> MHHHHHHPEIVDTCSLASPASVCRTKHLHLRCSVDFTRRTLTGTAALTVQSQEDNLRSLVLDTKDLTIEKVVINGQEVKYALGE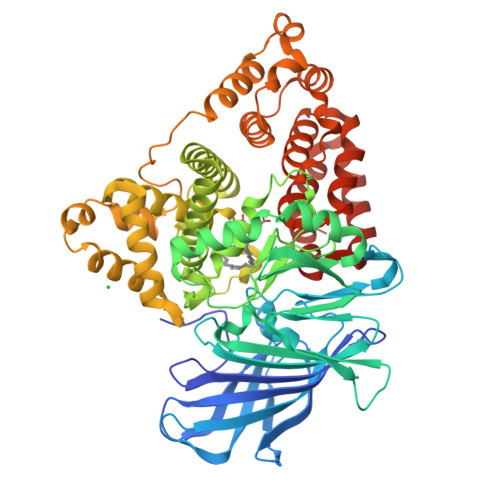RQSYKGSPMEISLPIALSKNQEIVIEISFETSPKSSALQWLTPEQTSGKEHPYLFSQCQAIHCRAILPCQDTPSVKLTYTAEVSVPKELVALMSAIRDGETPDPEDPSRKIYKFIQKVPIPCYLIALVVGALESRQIGPRTLVWSEKEQVEKSAYEFSETESMLKIAEDLGGPYVWGQYDLLVLPPSFPYGGMANPCLTFVTPTLLAGDKSLSNVIAHEISHSWTGNLVTNKTWDHFWLNEGHTVYLERHICGRLFGEKFRHFNALGGWGELQNSVKTFGETHPFTKLVVDLTDIDPDVAYSSVPYEKGFALLFYLEQLLGGPEIFLGFLKAYVEKFSYKSITTDDWKDFLYSYFKDKVDVLNQVDWNAWLYSPGLPPIKPNYDMTLTNACIALSQRWITAKEDDLNSFNATDLKDLSSHQLNEFLAQTLQRAPLPLGHIKRMQEVYNFNAINNSEIRFRWLRLCIQSKWEDAIPLALKMATEQGRMKFTRPLFKDLAAFDKSHDQAVRTYQEHKASMHPVTAMLVGKDLKVD> MAELACFCYPHLENDSYKFIPFNNLAIKAMLTAKVDKKDMDKFYDSIIYGIAPPPQFKKRYNTNDNSRGMNFETIMFTKVAMLICEALNSLKVTQANVSNVLSRVVSIRHLENLVIRKENPQDILFHSKDLLLKSTLIAIGQSKEIETTITAEGGEIVFQNAAFTMWKLTYLEHQLMPILDQNFIEYKVTLNEDKPISDVHVKELVAELRWQYNKFAVITHGKGHYRIVKYSSVANHADRVYATFKSNVKTGVNNDFNLLDQRIIWQN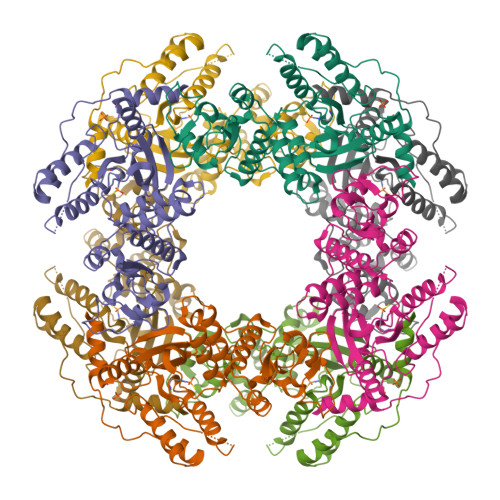WYAFTSSMKQGNTLDVCKRLLFQKMKPEKNPFKGLSTDRKMDEVSQVGV> LPTSNPAQELEARQLGRTTRDDLINGNSASCADVIFIYARGSTETGNLGTLGPSIASNLESAFGKDGVWIQGVGGA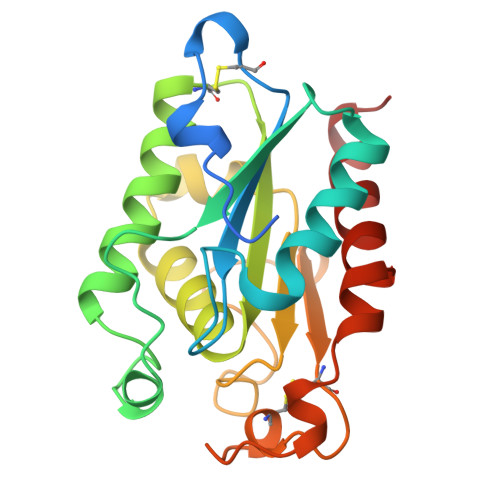YRATLGDNALPRGTSSAAIREMLGLFQQANTKCPDATLIAGGYSQGAALAAASIEDLDSAIRDKIAGTVLFGYTKNLQNLGRIPNYPADRTKVFCNTGDLVCTGSLIVAAPHLAYGPDARGPAPEFLIEKVRAVRGSA> GAQVSSQKVGAHENSNRAYGGSTINYTTINYYRDSASNAASKQDFSQDPSKFTEPIKDVLIKTAPMLNSPNIEACGYSDRVLQLTLGNSTITTQEAANSVVAYGRWPEYLRDSEANPVDQPTEPDVAACRFYTLDTVSWTKESRGWWWKLPDALRDMGLFGQNMYYHYLGRSGYTVHVQCNASKFHQGALGVFAVPEMCLAGDSNTTTMHTSYQNANPGEKGGTFTGTFTPDNNQTSPARRFCPVDYLLGNGTLLGNAFVFPHQIINLRTNNCATLVLPYVNSLSIDSMVKHNNWGIAILPLAPLNFASESSPEIPITLTIAPMCCEFNGLRNITLPRLQ;> GLGQMLESMIDNTVRETVGAATSR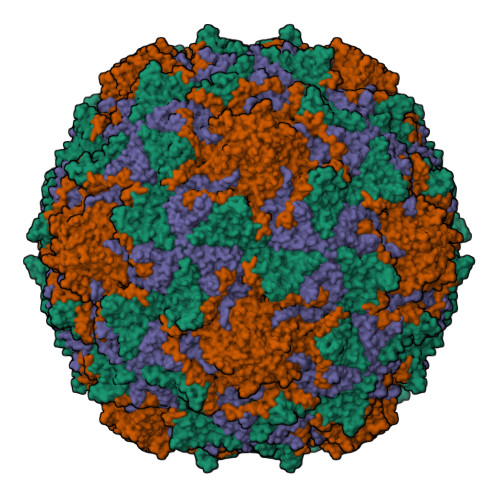DALPNTEASGPTHSKEIPALTAVETGATNPLVPSDTVQTRHVVQHRSRSESSIESFFARGACVTIMTVDNPASTTNKDKLFAVWKITYKDTVQLRRKLEFFTYSRFDMELTFVVTANFTETNNGHALNQVYQIMYVPPGAPVPEKWDDYTWQTSSNPSIFYTYGTAPARISVPYVGISNAYSHFYDGFSKVPLKDQSAALGDSLYGAASLNDFGILAVRVVNDHNPTKVTSKIRVYLKPKHIRVWCPRPPRAVAYYGPGVDYKDGTLTPLSTKDLTTY;> GLPVMNTPGSNQYLTADNFQSPCALPEFDVTPPIDIPGEVKNMMELAEIDTMIPFDLSATKKNTMEMYRVRLSDKPHTDDPILCLSLSPASDPRLSHTMLGEILNYYTHWAGSLKFTFLFCGSMMATGKLLVSYAPPGADPPKKRKEAMLGTHVIWDIGLQSSCTMVVPWISNTTYRQTIDDSFTEGGYISVFYQTRIVVPLSTPREMDILGFVSACNDFSVRLLRDTTHIEQKALAQ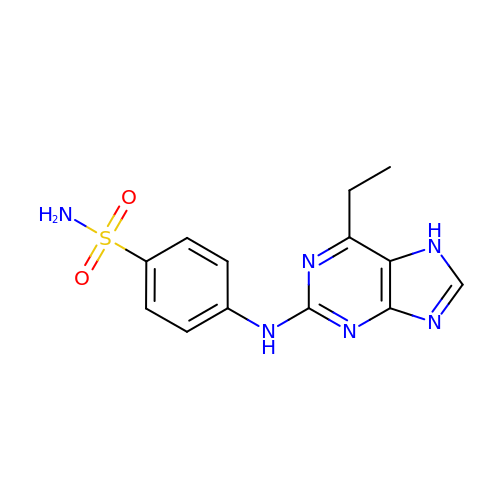4-[(6-ethyl-7~{H}-purin-2-yl)amino]benzenesulfonamide | C13 H14 N6 O2 S | UZLCQAXOQKFVGP-UHFFFAOYSA-N> TMRITKVEVDRKKVLISRDKNGGKLVYENEMQDNTEQIMHHKKSSFYKSVVNKTICRPEQKQMKKLVHGLLQENSQEKIKVSDVTKLNISNFLNHRFKKSLYYFPENSPDKSEEYRIEINLSQLLEDSLKKQQGTFICWESFSKDMELYINWAENYISSKTKLIKKSIRNNRIQSTESRSGQLMDRYMKDILNKNKPFDIQSVSEKYQLEKLTSALKATFKEAKKNDKEINYKLKSTLQNHERQIIEELKENSELNQFNIEIRKHLETYFPIKKTNRKVGDIRNLEIGEIQKIVNHRLKNKIVQRILQEGKLASYEIESTVNSNSLQKIKIEEAFALKFINACLFASNNLRNMVYPVCKKDILMIGEFKNSFKEIKHKKFIRQWSQFFSQEITVDDIELASWGLRGAIAPIRNEIIHLKKHSWKKFFNNPTFKVKKSKIINGKTKDVTSEFLYKETLFKDYFYSELDSVPELIINKMESSKILDYYSSDQLNQVFTIPNFELSLLTSAVPFAPSFKRVYLKGFDYQNQDEAQPDYNLKLNIYNEKAFNSEAFQAQYSLFKMVYYQVFLPQFTTNNDLFKSSVDFILTLNKERKGYAKAFQDIRKMNKDEKPSEYMSYIQSQLMLYQKKQEEKEKINHFEKFINQVFIKGFNSFIEKNRLTYICHPTKNTVPENDNIEIPFHTDMDDSNIAFWLMCKLLDAKQLSELRNEMIKFSCSLQSTEEISTFTKAREVIGLALLNGEKGCNDWKELFDDKEAWKKNMSLYVSEELLQSLPYTQEDGQTPVINRSIDLVKKY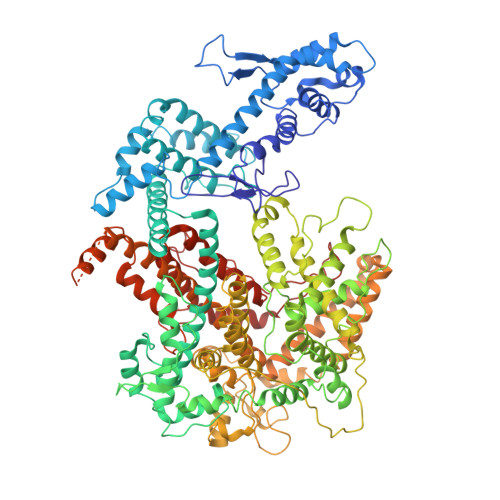GTETILEKLFSSSDDYKVSAKDIAKLHEYDVTEKIAQQESLHKQWIEKPGLARDSAWTKKYQNVINDISNYQWAKTKVELTQVRHLHQLTIDLLSRLAGYMSIADRDFQFSSNYILERENSEYRVTSWILLSENKNKNKYNDYELYNLKNASIKVSSKNDPQLKVDLKQLRLTLEYLELFDNRLKEKRNNISHFNYLNGQLGNSILELFDDARDVLSYDRKLKNAVSKSLKEILSSHGMEVTFKPLYQTNHHLKIDKLQPKKIHHLGEKSTVSSNQVSNEYCQLVRTLLTMK> MLIPAQENNVSLTATPSRIGQIMKYGFPGLDHVRSH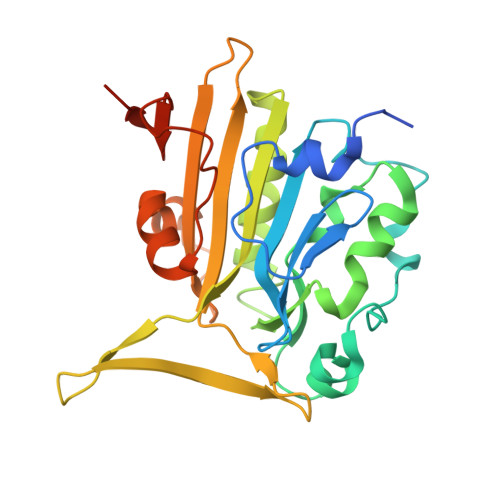SDYVLSYDRRNRVPHWVFEHLTAESVAKNDAVDRSKCDFKQDESIHPFFRSQNTDYRRSGYDRGHMAAAGNHRLHQKHCDETFYLSNMAPQVGQGFNRDAWNTLEAHVRRLTKTYSNVYVCTGPLYLPHKEDDGKSYVKYEVIGANTVAVPTHFYKVIVGESADHKLHMESYVMPNQVISNDTPISVFQVPPESVERSAGLLFFDQINRKQLTTINGKKVAAALEHHHHHH>MGSSHHHHHHSSENLYFQGGGHMTIDIGAGKLLAQEPTCPRDADGRPRVFVEGSGAYLTDPDGRRWIDFDNARGSVVLGHGDEEVAEAIARAARGRSGVGTAWSPVLDSLLGQLQEVCGGDVVGLYRTGTAALRSVTCAVRDARDRSIVLSSGYHGYDPMWHCDEPFTPNQHGIVEFLFDLDVLAEWLSRPEQVAAVVISPDHMHLGERWYTEFTRLTKEADVPVIADEVKVGLRYRAGLSTPLLDPAVWIVAKCLANGSPVAAVGGDAHLLAALEDVSFTSYFEPTAMAAATTTLRRMATGEPQQAIRAAGDRFIAHTRAAFANAGVPIDLAGNGNLFQFVCADDEVADAFHAAAAAEGLLFFEGDNQ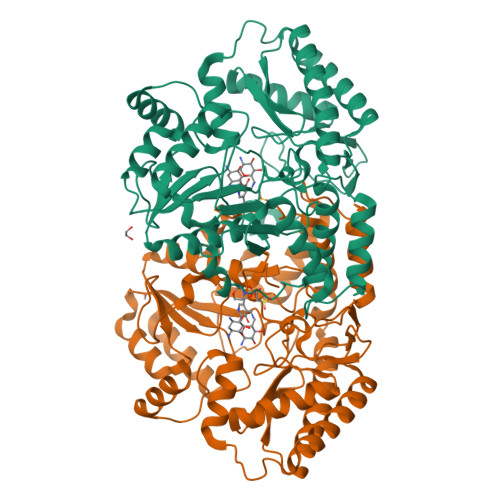TPSAAFTDEVVEDACGRIDRVSAALTGRFTDRELTEESWYASAWGAMDGLADRPRTREETTAIVERLWED[4x]> VPATRILLLVLAVIIYGTAGF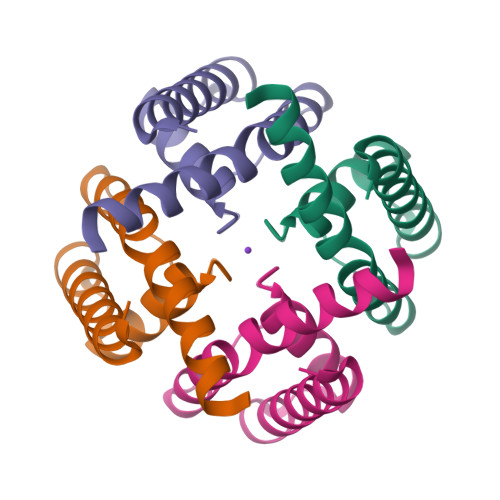HFIEGESWTVSLYWTFVTIATVGYGDYSPHTPLGMYFTCTLIVLGIGTFAVAVERLLEFLI>MNTVRSEKDSMGAIDVPADKLWGAQTQRSLEHFRISTEKMPTSLIHALALTKRAAAKVNEDLGLLSEEKASAIRQAADEVLAGQHDDEFPLAIWQTGSGTQSNMNMNEVLANRASELLGGVRGMERKVHPNDDVNKSQSSNDVFPTAMHVAALLALRKQLIPQLKTLTQTLNEKSRAFADIVKIGRTHLQDATPLTLGQEISGWVAMLEHNLKHIEYSLPHVAELALGGTAVGTGLNTHPEYARRVADELAVITCAPFVTAPNKFEALATCDALVQAHGALKGLAASLMKIANDVRWLASGPRCGIGEISIPENEPGSSIMPGKVNPTQCEALTMLCCQVMGNDVAINMGGASGNFELNVFRPM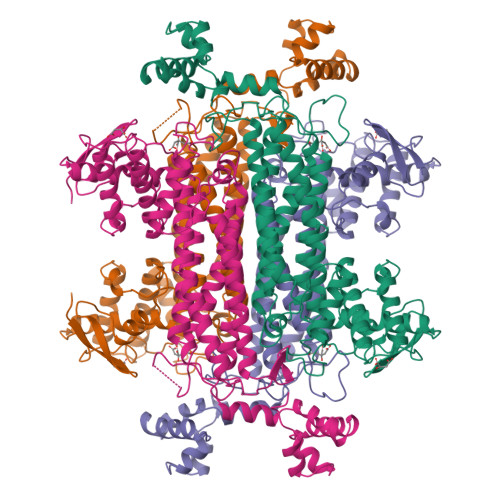VIHNFLQSVRLLADGMESFNKHCAVGIEPNRERINQLLNESLMLVTALNTHIGYDKAAEIAKKAHKEGLTLKAAALALGYLSEAEFDSWVRPEQMVGSMKAGR[2x]Finally, L‐sorbosone is further converted into 2‐KLG by a NAD(P)+‐dependent L‐sorbosone dehydrogenase (SNDH). Sequence analysis showed that the SNDH of G. oxydans WSH‐004 belongs to the aldehyde dehydrogenase (ALDH) superfamily (ALDH‐SF). Like other members of ALDH‐SF, SNDH has three typical domains: bridging domain (Red), catalytic domain (Yellow), and cofactor binding domain (Green). The crystal structural analysis found that the SNDH could exist in two different catalytic loop conformations, i.e., the oxidizing SNDH (O‐SNDH) with a closed substrate pocket and the reducing SNDH (R‐SNDH) with an open substrate pocket.

To verify whether the formation of the disulfide bond is a key factor affecting the motion of the catalytic loop, the crystal structure of R‐SNDH was analyzed by adding dithiothreitol (DTT) to the crystallization conditions. As with the C296A mutant, R‐SNDH was also resolved in a homotetrameric state, and each subunit had the same mode of action as mutant C296A. As expected, R‐SNDH has an open substrate pocket, in which Cys295 and Cys296 cannot form the disulfide bond, the sulfhydryl of Cys296 toward to the cofactor pocket, which called ‘resting’ state, blocking the cofactor‐substrate‐channel. The pose of the cofactor NADP+ in R‐SNDH is different from that in C296A. In R‐SNDH, the nicotinamide ring of NADP+ is extends to a solvent region, this pose should be that the sulfhydryl of Cys296 blocks the cofactor‐substrate‐channel, causing the cofactor channel of SNDH to have no space for the nicotinamide ring of NADP+. In R‐SNDH, although the nicotinamide ring has a larger displacement, it still has a hydrogen bond with Glu294. The pyrophosphate part loses the interaction with Trp162, and forms a hydrogen bond with Gly239. In the structure of R‐SNDH, the nicotinamide ring of NADP+ cannot enter the cofactor pocket because the catalytic residue Cys296 occupies a part of the cofactor pocket, and Cys296 should be in a ‘resting’ state. In the mutant C296A, since Ala296 has no sulfhydryl groups, an enough space can be left for NADP+ to enter the substrate‐cofactor‐channel. This indicates that SNDH may first accept the substrate during the reaction, which makes the sulfhydryl group of Cys296 point to the substrate pocket. Due to the deflection of the sulfhydryl of Cys296, the nicotinamide ring of NADP+ can correctly enter the cofactor channel to complete the electron transfer.

>[4x]MNVVSKTVSLPLKPREFGFFIDGEWRAGKDFFDRSSPAHDVPVTRIPRCTREDLDEAVAAARRAFENGSWAGLAAADRAAVLLKAAGLLRERRDDIAYWEVLENGKPISQAKGEIDHCIACFEMAAGAARMLHGDTFNNLGEGLFGMVLREPIGVVGLITPWNFPFMILCERAPFILASGCTLVVKPAEVTSATTLLLAEILADAGLPKGVFNVVTGTGRTVGQAMTEHQDIDMLSFTGSTGVGKSCIHAAADSNLKKLGLELGGKNPIVVFADSNLEDAADAVAFGISFNTGQCCVSSSRLIVERSVAEKFERLVVAKMEKIRVGDPFDPETQIGAITTEAQNKTILDYIAKGKAEGAKLLCGGGIVDFGKGQYIQPTLFTDVKPSMGIARDEIFGPVLASFHFDTVDEAIAIANDTVYGLAASVWSKDIDKALAVTRRVRAGRFWVNTIMSGGPETPLGGFKQSGWGREAGLYGVEEYTQIKSVHIETGKRSHWISHHHHHH>DVPLTPSQFAKAKSENFDKKVILSNLNKPHALLWGPDNQIWLTERATGKILRVNPESGSVKTVFQVPEIVNDADGQNGLLGFAFHPDFKNNPYIYISGTFKNPKSTDKELPNQTIIRRYTYNKSTDTLEKPVDLLAGLPSSKDHQSGRLVIGPDQKIYYTIGDQGRNQLAYLFLPNQAQHTPTQQELNGKDYHTYMGKVLRLNLDGSIPKDNPSFNGVVSHIYTLGHRNPQGLAFTPNGKLLQSEQGPNSDDEINLIVKGGNYGWPNVAGYKDDSGYAYANYSAAANKSIKDLAQNGVKVAAGVPVTKESEWTGKNFVPPLKTLYTVQDTYNYNDPTCGEMTFICWPTVAPSSAYVYKGGKKAITGWENTLLVPSLKRGVIFRIKLDPTYSTTYDDAVPMFKSNNRYRDVIASPDGNVLYVLTDTAGNVQKDDGSVTNTLENPGSLIKFTYKAK[2x]

The soluble glucose dehydrogenase (sGDH) from Acinetobacter calcoaceticus has been widely studied and is used, in biosensors, to detect the presence of glucose, taking advantage of its high turnover and insensitivity to molecular oxygen. However, this dimeric enzyme, composed of two identical 453 amino acid monomers (pI = 8.75), also presents drawbacks in terms of broad substrate specificity and loss of activity over time. Briefly, all crystal structures contained a tight dimer of sGDH in the asymmetric unit, the dimeric interface extending over 1110 Å2 being maintained by the presence of two calcium ions as described in Oubrie et al. interacting with the N262-D273 loop, referred to as the 4CD loop in the nomenclature of Oubrie et al.. 2Fobs-Fcalc electron density maps from the wild-type and both mutant structures all showed a different molecule instead of the PQQ-cofactor, corresponding to a PQQ modified cofactor, with the bond between C4 and C5 missing.

We report the characterization of two sGDH mutants: the single mutant Y343F and the double mutant D143E/Y343F. The mutants present enzyme selectivity and specificity of 1.2 (Y343F) and 5.7 (D143E/Y343F) times higher for glucose compared with that of the wild-type. N428T and D143E mutations significantly reduced selectivity for lactose and maltose, with a cumulative effect for the double mutation D143E/N428T. The D143E/Y343F mutant presents a classical Michaelian behavior with both monomer sites equivalent and a single value of KM. For example, at physiological concentrations (5 mM), the Y343F and the D143E/Y343F mutants have a glucose oxidation steady-state catalytic rate constant (kss) 1.5 and 7.1 times increased compared with that of maltose, respectively. At pH 7.5, the addition of catalase slows down the aging of the enzyme. By consuming the H2O2 once it is produced, catalase indirectly maintains the integrity of the cofactor and compared with the enzyme without catalase, increases the retention of enzymatic activity of sGDH for at least 8 h. Numerous attempts to co-crystallize mutant protein with glucose and maltose substrates all failed to locate the sugar substrates in the resolved structures (data not shown). Indeed, as can be seen in Figure 4, the rotation of the pyrrole ring obscures the glucose binding site observed by Oubrie.Protein tyrosine phosphatases (PTPs) play a critical role in regulating cellular functions by selectively dephosphorylating their substrates. The ∼280 residue PTP catalytic domain consists of an α/β structure, and biochemical and structural studies have led to a detailed understanding of the catalytic mechanism (Barford et al., 1994; Zhang, 2002). Key features of the domain include the PTP signature motif, the mobile Trp-Pro-Asp “WPD” loop that in the closed conformation positions the conserved and catalytically important aspartate residue, and the phosphotyrosine recognition loop. Here we report the crystal structures of 22 PTP domains, including two tandem-domain RPTP structures and a detailed structural comparison of this protein family.

In the first category are TCPTP, SHP1, SHP2, BDP1, LYP, PEST, PTPBAS, DEP1, MEG2, and GLEPP1, which have a “PTP1B-like” accessible pocket that harbors a basic residue corresponding to Arg24 of PTP1B. This pocket has the potential to accommodate pY at the +1 position as in PTP1B or potentially other acidic or phosphorylated residues in positions N-terminal to the substrate pY. The new structural data and analysis presented here suggest that a secondary substrate-binding pocket, similar to that found in PTP1B, is present also in SHP2, BDP1, LYP, SHP1, TCPTP, MEG2, PTPBAS, DEP1, and GLEPP1. PTPs with particularly high enzymatic activity against generic substrates were RPTPσ and PTP subgroups R5, R3, NT1, NT2, NT3, NT4, and NT5. The subgroups NT1, NT2, NT3, and NT5 exhibited a pronounced preference for acidic residues N-terminal to the phosphorylation site.

>MSVHVPGPHAMTIQELVDYVNARQKQGIYEEYEDIRRENPVGTFHCSMSPGNLEKNRYGDVPCLDQTRVKLTKRSGHTQTDYINASFMDGYKQKNAYIGTQGPLENTYRDFWLMVWEQKVLVIVMTTRFEEGGRRKCGQYWPLEKDSRIRFGFLTVTNLGVENMNHYKKTTLEIHNTEERQKRQVTHFQFLSWPDYGVPSSAASLIDFLRVVRNQQSLAVSNMGARSKGQCPEPPIVVHCSAGIGRTGTFCSLDICLAQLEELGTLNVFQTVSRMRTQRAFSIQTPEQYYFCYKAILEFAEKEGMVSAHHHHHH[2x]> GSSGKRFVHVKNPYLDLMDEDILYHLDLGTKTHNLPAMFGDVKFVCVGGSPNRMKAFALFMHKELGFEEAEEDIKDICAGTDRYCMYKTGPVLAISHGMGIPSISIMLHELIKLLHHARCCDVTIIRIGTSGGIGIAPGTVVITDIAVDSFFKPRFEQVILDNIVTRSTELDKELSEELFNCSKEIPNFPTLVGHTMCTYDFYEGQGRLDGALCSFSREKKLDYLKRAFKAGVRNIEMESTVFAAMCGLCGLKAAVVCVTLL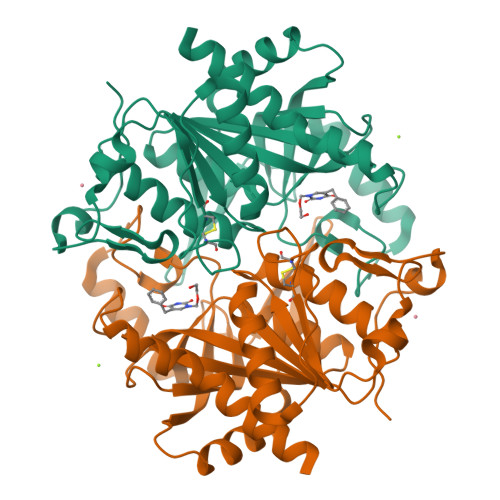DRLDCDQINLPHDVLVEYQQRPQLLISNFIRRRLG N-benzyl-2-[(N-benzylglycyl)amino]-4-phenylthiophene-3-carboxamide | C27 H25 N3 O2 S | 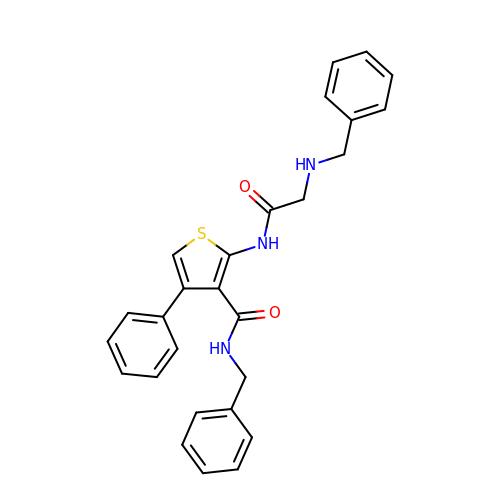FATCVHYQVCDDIO-UHFFFAOYSA-N> MELWLVRHGETLWNREGRLLGWTDLPLTAEGEAQARRLKGALPSLPAFSSD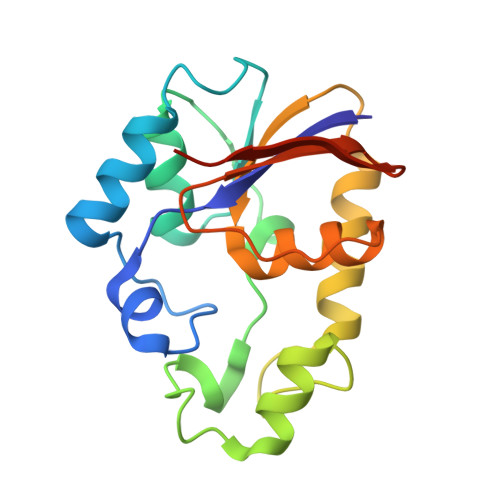LLRARRTAELAGFSPRMYPELREIHFGALEGALWETLDPRYKEALLRFQGFHPPGGESLSAFQERVFRFLEGLKAPAVLFTHGGVVRAVLRALGEDGLVPPGSAVAVDWPRRVLVRLALDGEEATG>[2x]MARARPSVAGGGVAAPPERAGPGRPRRSRTGHHCDPECPGLRAAPRTPGPGAGRRAAKLRPGRGWWALLLLQLHLLRALAQDDVAPYFKTEPGLPQIHLEGNRLVLTCLAEGSWPLEF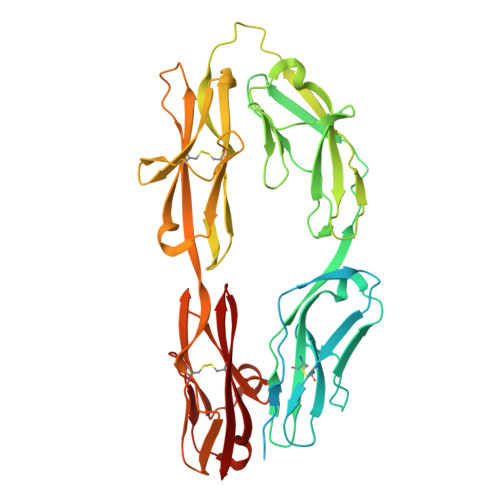KWIRNDSELTTYSSEYKYIIPSLQKLDAGFYRCVVRNRMGALLQRKSEIQVAYMGNFMDTDQRKTVSQGHAALLNLLPIVSCPQPQVTWFREGHKIIPSSRIAITLENQLVILATTASDAGAYYVQAVNEKNGENKTSPFIHLSVARDTGTHEAMAPIIVVAPGNRSVVAGSSETTLECIANARPVEELSVHWKRNGVRLTSGLHSYGRRLTITNPTSADTGMYVCEATLRGSTFEPARARAFLSIIEPPYFTAEPESRILGEVEETMDIPCRAMGVPLPTLQWYKDAVPLSKLQNPRYKVLPSGGLHIQKLSPEDSGIFQCFASNEGGEVQTHTYLDVT> GHMECIKGNVDLVFLFDGSMSLQPDEFQKILDFMKDVMKKLSNTSYQFAAVQFSTSYKTEFDFSDYVKRKDPDALLKHVKHMLLLTNTFGAINYVATEVFREELGARPDAT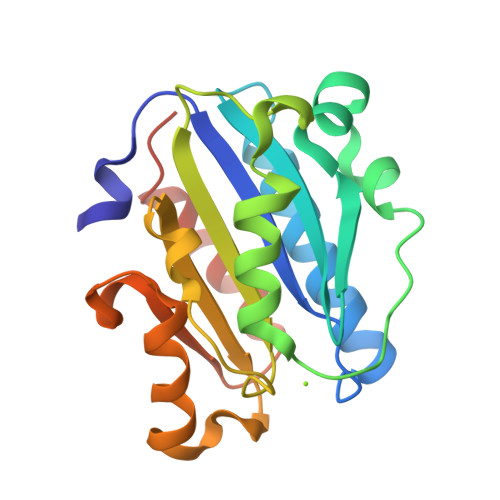KVLIIITDGEATDSGNIDAAKDIIRYIIGIGKHFQTKESQETLHKFASKPASEFVKILDTFEKLKDLFTELQKKIYVIEGTSKQD> MGSSHHHHHHSQDPMEIDELTALGGLLANIGKPVQRAGLYSGDHSTQGARFLRDLAENTGRAEYELLSLFSEFHHKGHMKNDELMIRRIKELSPERFGLTMEDVLNALWIVYEADNLASGEREEGQPQASRPLYSVFNPGKAYPWAELDFEKELPVPGDVFSIRSQDYRELVKRLWEELSKAKLRSDRLLPVLEKYLTFVSSVTSEGNIISLYDHMRMTSAIALAMLRAGCTAEDVRSGRCRKEKRFLLIEGDFSGIQDFIYRVSGKGTLKYLRARSAYLELIGWDVVLEILSRLGLTRANVVFNAGGHFMIIAQNTPDAVKELEEIRAKAVEWLYREFESDLYLAIEWEPVSGREFGREGGKNLFAEARKRLKHKLTVRKLKRFGEIKGLFEHGHTERLAECPVCGRELPEGKLEPSASDPETKVCPTCNRLVSLGGNLPKLLGFGRTAKNDAGVLVEGPFSGFVPYLQGGRPVGEQILVKNTLNPGEIPESAQFVPYFVADYFKKDPKGGVATFEELSMASTGTRRLGVMKGDVDRLGEFFSSMDSPSKLATASRFMDYFFKGYIGAIIEGKFGYIIGDVPSLRDWPEEPDIVVVYAGGDDFFIVGAWDQIFELAFRVRRAFNAYTGGKLTLSVGLGYFDERTPIYRMADVVSERLDTAKDEGRNRVFVVGRSRPLDGKHKLSYEWNHYEELWRTYAPRIYAGNGRLKGKLESKKGLLWKLLEIRELYVRDPNDVRWAYLTAYLLGRHGLSDLFPELVGIDTKAVERKEPQPVYWVDGVLKIVLMAVRR;> SMAYHQKHGGYGRGGYGRQDRPQVDASRLFGESPDVVGIKKMLEGKGKQWEAIQPYFDNVVREAKNFLEWSPNKRLANAVTVAAYLTSQGLKTNQVRKILDMARTTELKVKRGEGDIKDDLVKMRYLLAYTVGKATGQSKYSLDAFHRILDPMLEVLMGSPKKENFEKFYDFLQAVVAYHKFFGGGD;>SMDRRFYGKIVIKGKIKAVTGLHIGSQRDISEIGGIANPVIKDPHTGLPYIPGSSLKGRLRSLFEILVNSRLGEWREKYPSLANYSPGSCRPDNQENCGKFFNRKINRGWIHVCPDYETALACPVCRLFGASGKESNFPSRIIVRDAFLTKEWEEKWRAGEAITEAKIEVGIDRVTSQANPRTNERVVAGAEFEFEIIYNVENTTHWRDDIKNLLTAMALLEDSYLGGSGSRGYGKVKFIFDSFEFRPLDYYRTGKDEDIVSIDAREKSVSDILSGFDSLFSEVEGKLEAG[2x];> MPKFIAVKLIPKGPFRDIPR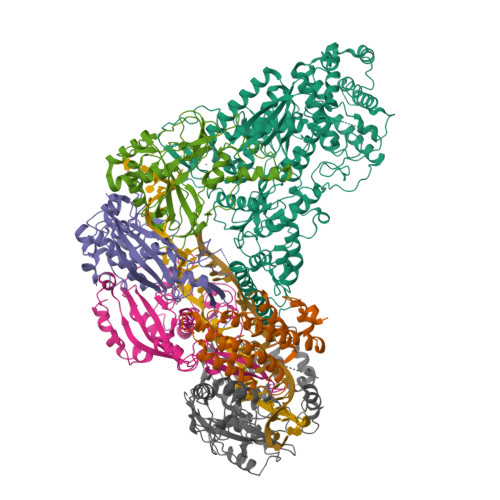ADTLFGAIGNAISAIHGQSAVEELVDAFVGGARISSAFPYSGDTYYLPKPLSVEPALEGILTGLDEEERYTTAKRLRKAKYLDLKNFELALRLRPFTIPEEIPYARVDVPRVVLDRVTQDSSIYFWEEIRFREKSGVYFLYSGPREVFDGYIAPAMRFLGDTGIGGKSTWGAGLFEVEFHEMKIDAPGSEYSVTLSNALPTKTPVLWRLLRKGGWSFGRRKPRMTFIAEGSIVKNDPGGMERLELGLSHEVYVYGLTFPLGVELPEGLE;> MTERTLKVLSPLHIGTGNELTPVDIYPRENIIHVLDTERLVNDLMNLGVELNEILALLKNPPGDAYIWKGYIEEFHLDPSDYSIYTLKIHGKIGRKSMQIKEFIKLNGRPYIPGSSLKGAIRTAVLYKALKECGDARAVMRVVSKVNGDVARDIGRSEDVLDYYMSFLSRARIDRKRADDLLEAIVFGMEPDRRSKIRYEPKRDPMKALIVRDSKPVGRKHLAVYHVEVIGNPQPIPIWVEAIEPGAATDVEIHVDTEALRLNADYFNGLLWECLKERGEPGEVFEDFLWEAVDEFYTAVMKYETIEVQKFGRYTSQVRSFYASLEDHSGHVLRLGWGSGWLAMTIGLLLVEKGYKWENVRKKLGLGKKPGGSGFSREFPKTRRLADGMPMGWVVLEHHHHHH> GSMKKERVITEFWDGKIIMVSPDDPKYALKKAEEVRELVDSELGFQQVSLRCPSQTRTYMFVSNEKKIVGCLIAEPIREAYRVLA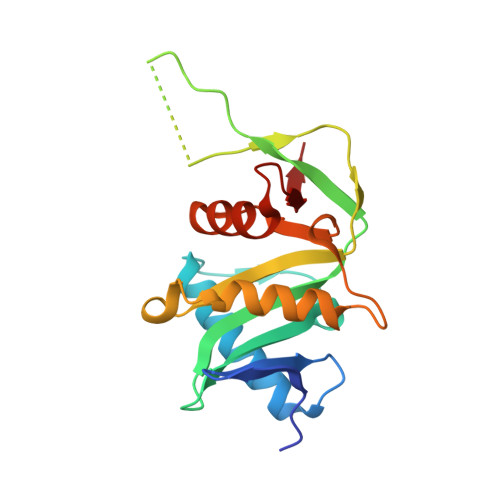EPPSLHSLHGEPLERHRAWRCSTEPEPAICGISRIWVFALMRRKAIASRMVDAVRSSFMYGSVLTTEEIAFSDPTPDGKLFASTYCKVPDFLVYNFVS> TIQPGTGYNNGYFYSYWNDGHGGVTYTNGPGGQFSVNWSNSGNFVGGKGWQPGTKNKVINFSGSYNPNGNSYLSVYGWSRNPLIEYYIVENFGTYNPSTGATKLGEVTSDGSVYDIYRTQRVNQPSIIGTATFYQYWSVRRNHRS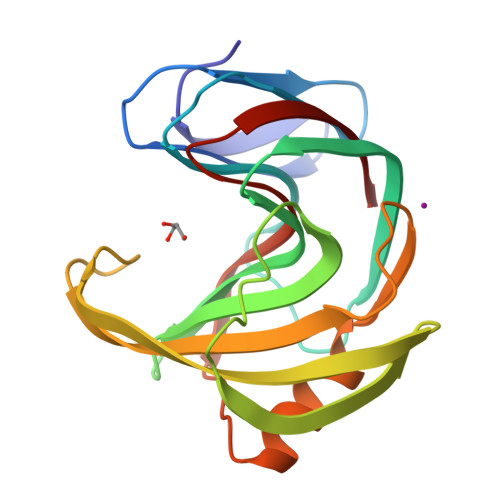SGSVNTANHFNAWAQQGLTLGTMDYQIVAVEGYFSSGSASITVS>[3x]GG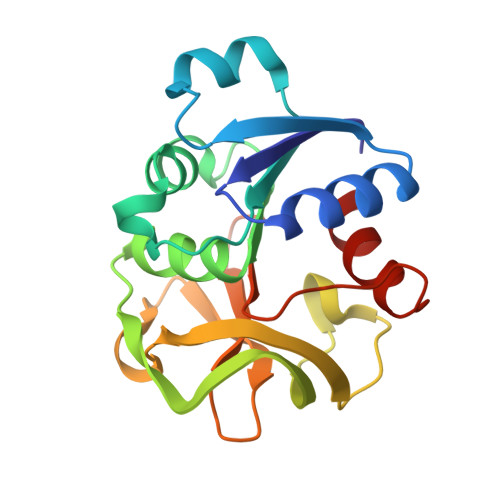MILLIDNYDSFTWNLYQYFCELGADVLVKRNDALTLADIDALKPQKIVISPGPCTPDEAGISLDVIRHYAGRLPILGVCLGHQAMAQAFGGKVVRAAKVMHGKTSPITHNGEGVFRGLANPLTVTRYHSLVVEPDSLPACFDVTAWSETREIMGIRHRQWDLEGVQFHPESILSEQGHQLLANFLHR>GPLGSSLHIYNWTDYIAPTTLKDFTKESGIDVSYDVFDSNETLEGKLVSGHSGYDIVVPSNNFLGKQIQAGAFQKLDKSKLPNWKNLDPALLKQLEVSDPGNQYAVPYLWGTNGIGYNVAKVKEVLGDQPIDSWAILFEPENMKKLAKCGVAFMDSGDEMLPAALNYLGLDP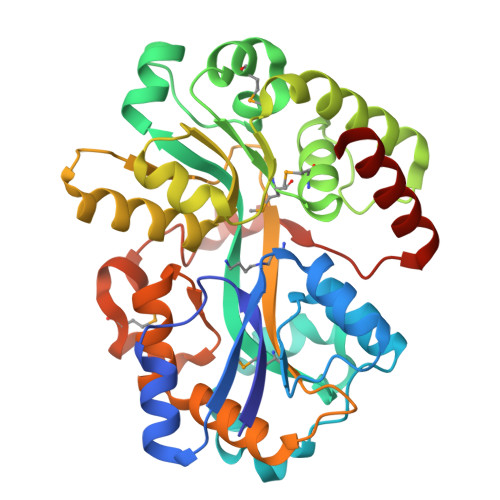NTHDPKDYKKAEEVLTKVRPYVSYFHSSKYISDLANGNICVAFGYSGDVFQAAARAEEAGKGIDIQYVIPKEGANLWFDLMAIPADAKAADNAYAFIDYLLRPEVIAKVSDYVGYANAIPGARPLMDKSVSDSEEVYPPQAVLDKLYVSAVLPAKVLRLQTRTWTRIK[2x]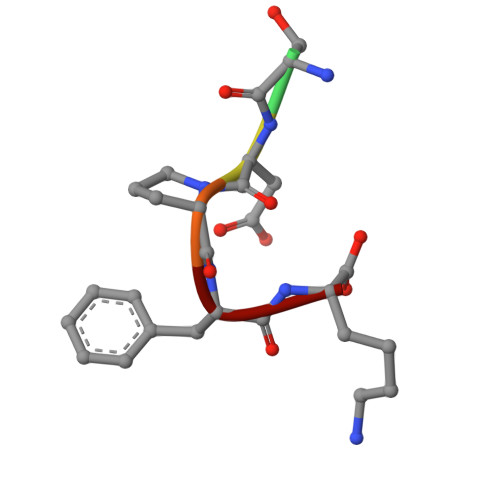> GSDPFK> GASQFFKDNCNRTTASLVEGVELTKYISDINNNTDGMYVVSSTGGVWRISRAKDYPDNVMTAEMRKIAXAAVLSGMRVNMCASPASSPNVIWA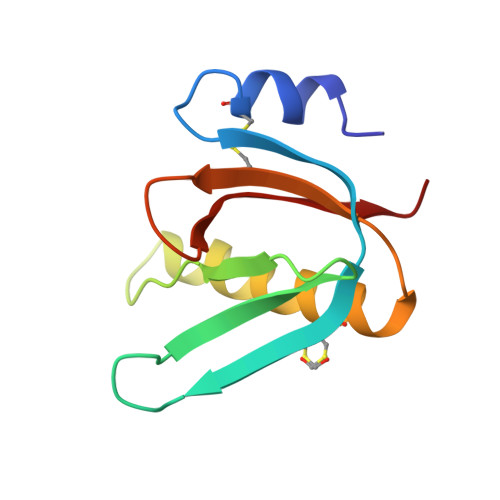IELEAE>[2x]FVLTEGNPRWEQTHLTYRIENYTPDLPRADVDHAIEKAFQLWSNVTPLTFTKVSEGQADIMISFVRGDHRDNSPFDGPGGNLAHAFQPGPGIGGDAHFDEDERWTNNFREYNLHRVAAHALGHSLGLSHSTDIGALMYPSY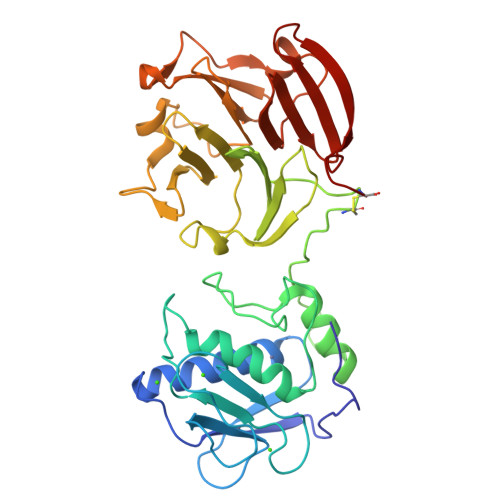TFSGDVQLAQDDIDGIQAIYGRSQNPVQPIGPQTPKACDSKLTFDAITTIRGEVMFFKDRFYMRTNPFYPEVELNFISVFWPQLPNGLEAAYEFADRDEVRFFKGNKYWAVQGQNVLHGYPKDIYSSFGFPRTVKHIDAALSEENTGKTYFFVANKYWRYDEYKRSMDPGYPKMIAHDFPGIGHKVDAVFMKDGFFYFFHGTRQYKFDPKTKRILTLQKANSWFNC> MAGGEAGVTLGQPHLSRQDLTTLDVTKLTPLSHEVI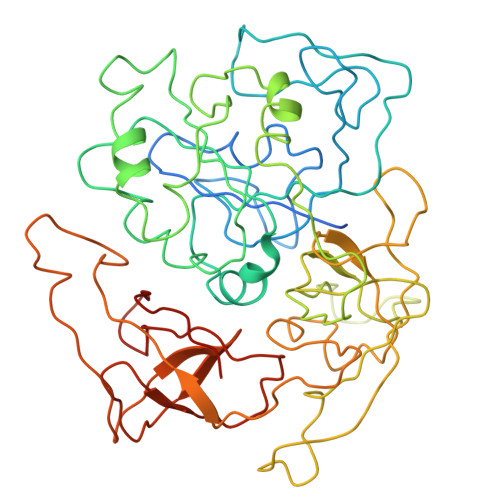SRQATINIGTIGHVAHGKSTVVKAISGVHTVRFKNELERNITIKLGYANAKIYKLDDPSCPRPECYRSCGSSTPDEFPTDIPGTKGNFKLVRHVSFVDCPGHDILMATMLNGAAVMDAALLLIAGNESCPQPQTSEHLAAIEIMKLKHILILQNKIDLVKESQAKEQYEQILAFVQGTVAEGAPIIPISAQLKYNIEVVCEYIVKKIPVPPRDFTSEPRLIVIRSFDVNKPGCEVDDLKGGVAGGSILKGVLKVGQEIEVRPGIVSKDSEGKLMCKPIFSKIVSLFAEHNDLQYAAPGGLIGVGTKIDPTLCRADRMVGQVLGAVGALPEIFTELEISYFLLRRLLGVRTEGDKKAAKVQKLSKNEVLMVNIGSLSTGGRVSAVKADLGKIVLTNPVCTEVGEKIALSRRVEKHWRLIGWGQIRRGVTIKPTVDDD> THWFHRNPLKATAPVSFNYYGVVTGPSASKICNDLRSSRARLLELFTDLSCNPEMMKNAADSYFSLLQGFINSLDESTQESKLRYIQNFKWTDTLQGQVPSAQQDAVFELISMGFNVALWYTKYASRLAGKENITEDEAKEVHRSLKIAAGIFKHLKESHLPKLITPAEKGRDLESRLIEAYVIQCQ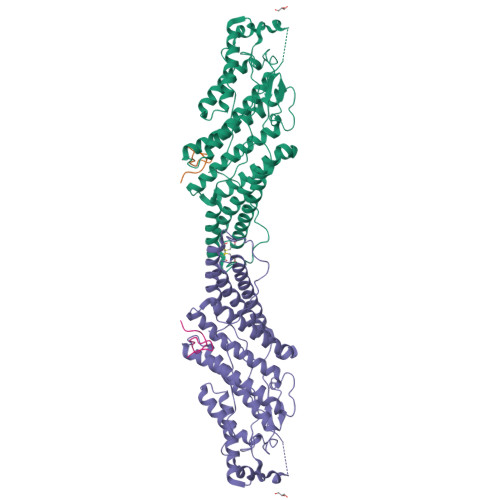AEAQEVTIARAIELKHAPGLIAALAYETANFYQKADHTLSSLEPAYSAKWRKYLHLKMCFYTAYAYCYHGETLLASDKCGEAIRSLQEAEKLYAKAEALCKEYGETKGPGPTVKPSGHLFFRKLGNLVKNTLEKCQRENGFIYFQKIPTEAPQLELKANYGLVEPIPFEFPPTSVQWTPETLAAFDLTKRPKDDSTKPKPEEEVKPVKEPDIKPQKDTGCYIS;> RSYGTPELDEDDLEAELDALGDELLADEDSSYLDEAASAPAIPEGVPTDTKNKDGVLVDEFGLPQIPAS2-ETHYLIMIDAZOLE | C5 H8 N2 | 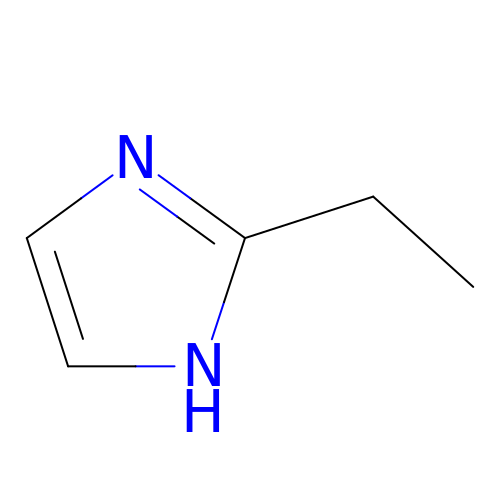PQAMFDRRWURCFQ-UHFFFAOYSA-N4-{5-[(4-hydroxyphenyl)amino]-1H-pyrazol-3-yl}phenol | C15 H13 N3 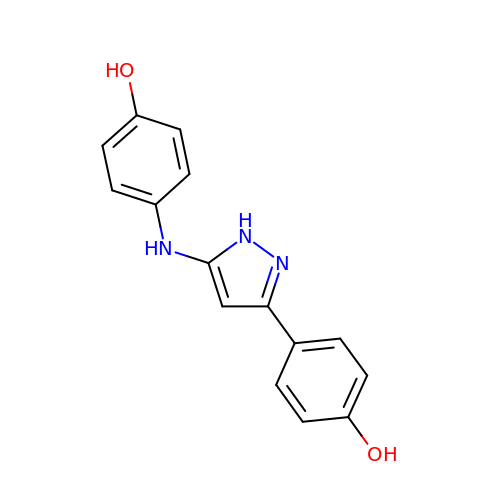O2 | AWPPGEGXTUMWMX-UHFFFAOYSA-N> MTTACPARTSSLMDDLLGLLRIRIKRGVNLAVRDISSSDPYVVVKMGKQKLKTRVINKDVNPEWNEDLTLSVTDSNLTVLLTVYDHDMFSKDDKMGDAEFEISPYIEALRMQLDGLPSGTIVTTVKPSRRNCLAEESRVTWVDGKLVQDLVLRLRHVECGEVEAQLQWIDLPGSKGL;> MTTACPARTSSLMDDLLGLLRIRIKRGVNLAVRDISSSDPYVVVKMGSQKLKTRVINKDVNPEWNEDLTLSVTDSNLTVLLTVYDHDMFSKDDKMGDAEFEIKPYIEALRMQLGGLPSGTIVTTVKP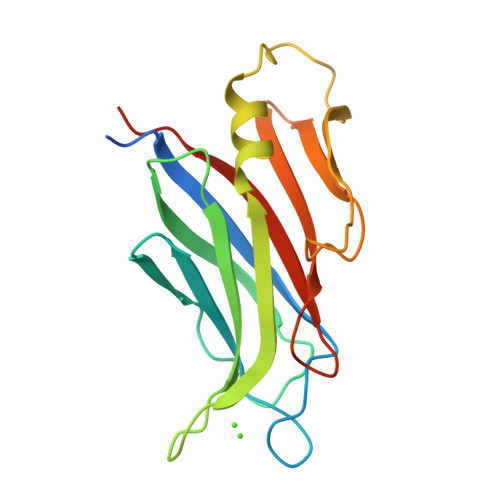SRRNCLAEESRVTWVDGKLVQDLVLRLRHVECGEVEAQLQWIDLPGSSGL> MSPVFTNSTYTVLVEENLPAGTTILQIEAKDVDLGANVSYRIRSPEVKHFFALHPFTGELSLLRSLDYEAFPDQEASITFLVEAFDIYGTMPPGIATVTVIVKDMNDYPPVFSKRIYKGMVAPDAVKGTPITTVYAEDADPPGLPASRVRYRVDDVQFPYPASIFEVEEDSGRVITRVNLNEEPTT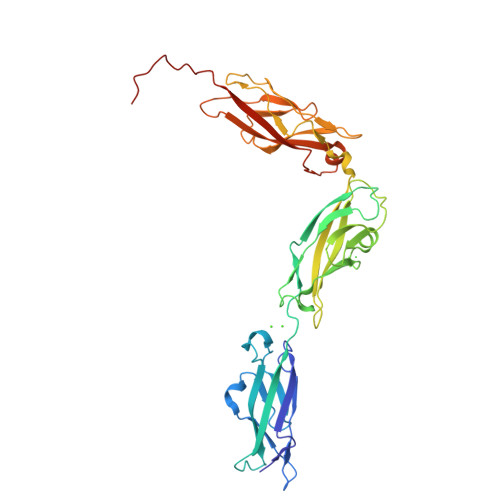IFKLVVVAFDDGEPVMSSSATVKILVLHPGEIPRFTQEEYRPPPVSELATKGTMVGVISAAAINQSIVYSIVSGNEEDTFGINNITGVIYVNGPLDYETRTSYVLRVQADSLEVVLANLRVPSKSNTAKVYIEIQDENNHPPVFLEHHHHHH>[8x]SMLTELIASNRRSAAIHAFVDTGLSTHFKDGIYVDISELSRKSGVNYARFSRLCDFLVEMGVLVSNDNKFRLSDECHVFANPESFESFMIKLEICSHYSNAWLMYGKSLFEDDGKSAFEMAHGRPFFEYLDGNKFLKSNFDALMTRVSNLIVEKLLGIYDFNQHNRILDVGGGEGELLVRISEKVKGKHYAVLDRYSELPVSDNIDFIN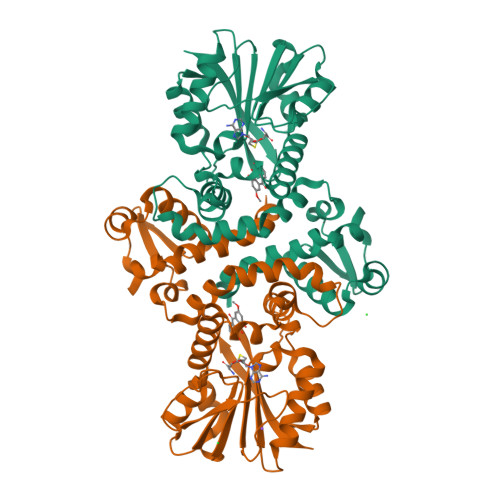GNFLNSIPSGYDLYILKNVLHNWSDSDSILILENFRKAMDKNSSLLLINMVKEPEFSRSFDILMDVLFLGKERSFTEFEYLANQAGLVVQETKVIDQSYSPYSFIKLQIK>GSDPQVLRGSGHCKWFNVRMGFGFISMTSREGSPLENPVDVFVHQSKLYMEGFRSLKEGEPVEFTFKKSSKGFESLRVTGPGGN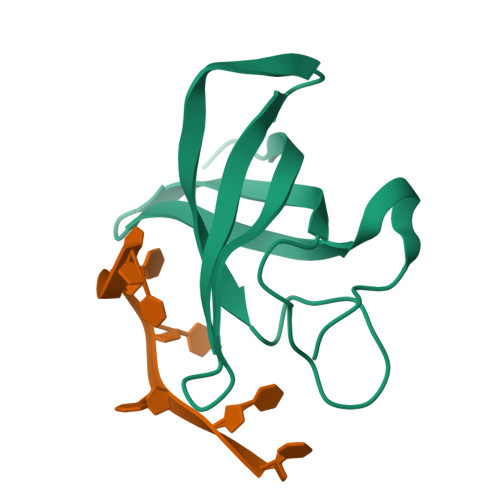PCLGNE[4x]> SAAPSVFLIDDDRDLRKAMQQTLELAGFTVSSFASATEALAGLSADFAGIVISDIRMP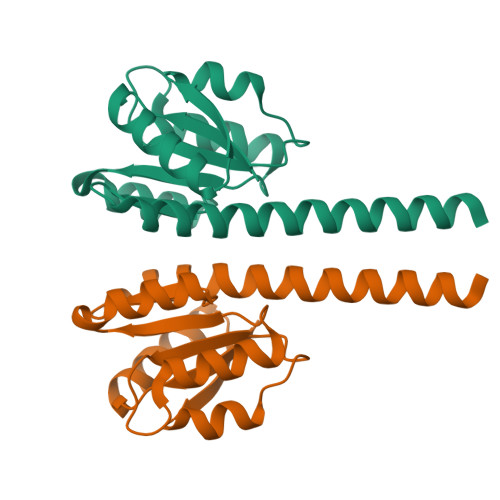GMDGLALFRKILALDPDLPMILVTGHGDIPMAVQAIQDGAYDFIAKPFAADRLVQSARRAEEKRRLVMENRSLRRAAEAASEGLKLAAALEHHHHHH>GSMHARIVERPAFSVVGMEYFGSAPGDTIGQLWERFIPREHEIAGKHDPEVSYGICAQQPNGEFHYVAGFEVQEGWPVPEGMVRFQVPAQKYAVFTHKGTAPQIAESFQAIYSHLLAERGLEPKAGVDFEYYDQR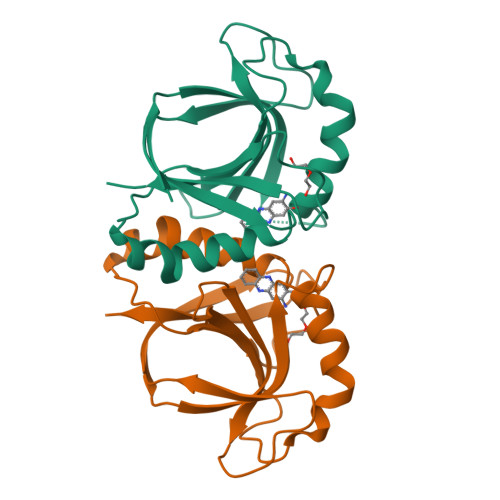FRGPLDPNSQVDLYIPIY[2x]CYCLOPENTANECARBOXYLIC ACID 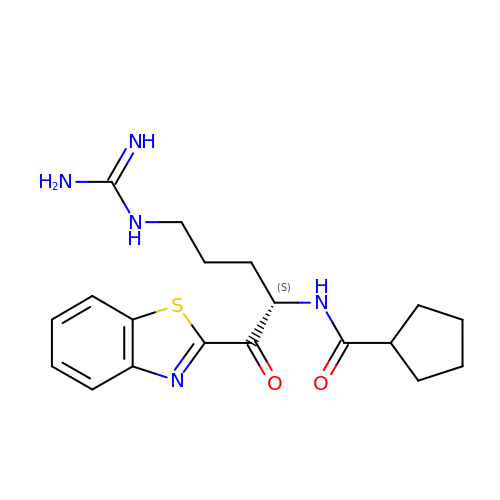[1-(BENZOTHIAZOLE-2-CARBONYL)-4-GUANIDINO-BUTYL]-AMIDE | C19 H25 N5 O2 S | NQABUEUFRXDDFI-AWEZNQCLSA-N> MGHHHHHHGSMALPKDAIPSLSECQCGICMEILVEPVTLPCNHTLCKPCFQSTVEKASLCCPFCRRRVSSWTRYH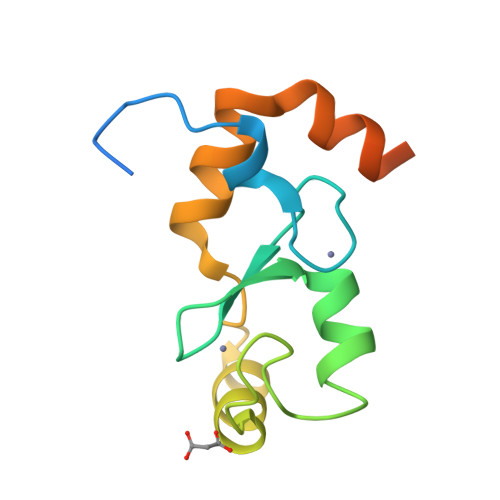TRRNSLVNVELWTIIQKHYPRECKLRASGQESEEVADDYQPVRLLS> LYFQGAMALEEIKNGTDISTLDIRKFNLNINNVSVLSKSQSVDQFHLSNPHYEYLSGGAYPGEMENFTLKVDKSKKQDQVFENPLSLKFTNIGTVNGKQVDAYLNFNKVTLHYLNTAQAESEMNSAQKSTVEFFSISELWESNAFEIGNVPYVDANHDYIMNKAFWIDADVTAEIRYADGTETDLKLVMKPTDIDAIDANNLKETFYVKNYQNDVNLRLMNNANVLVQEEASDRTSWIATQITGGSYNENNVSGLALRSNSNSMNFGYSSTETCSAVFGLYIEKIDPRPVLEVDPAEIPAKDGQDVTYKATFKVPVPGKDILAAPSSIEMVQKFDERLDYKELKVESGGVTLQEGRDYTIEKTGQTVTVKMTPEYLKGNSSSDIIITYKTATNKKVEEKGSEKIDNTVTLHVDNLSAPSNQVSTALLYEK;> PTTENLYFQGAMALEEIKNGTDISTLDIRKFNLNINNVSVLSKSQSVDQFHLSNPHYEYLSGGAYPGEMENFTLKVDKSKKQDQVFENPLSLKFTNIGTVNGKQVDAYLNFNKVTLHYLNTAQAESEMNSAQKSTVEFFSISELWESNAFEIGNVPYVDANHDYIMNKAFWIDADVTAEIRYADGTETDLKLVMKPTDIDAIDANNLKETFYVKNYQNDVNLRLMNNANVLVQEEASDRTSWIATQITGGSYNENNVSGLALRSNSNSMNFGYSSTETCSAVFGLYIEKIDPRPVLEVDPAEIPAKDGQDVTYKATFKVPVPGKDILAAPSSIEMVQKFDERLDYKELKVESGGVTLQEGRDYTIEKTGQTVTVKMTPEYLKGNSSSDIIITYKTATNKKVEEKGSEKIDNTVTLHVDNLSAPSNQVSTALLYEK;> IPTTENLYFQGAMALEEIKNGTDISTLDIRKFNLNINNVSVLSKSQSVDQFHLSNPHYEYLSGGAYPGEMENFTLKVDKSKKQDQVFENPLSLKFTNIGTVNGKQVDAYLNFNKVTLHYLNTAQAESEMNSAQKSTVEFFSISELWESNAFEIGNVPYVDANHDYIMNKAFWIDADVTAEIRYADGTETDLKLVMKPTDIDAIDANNLKETFYVKNYQNDVNLRLMNNANVLVQEEASDRTSWIATQITGGSYNENNVSGLALRSNSNSMNFGYSSTETCSAVFGLY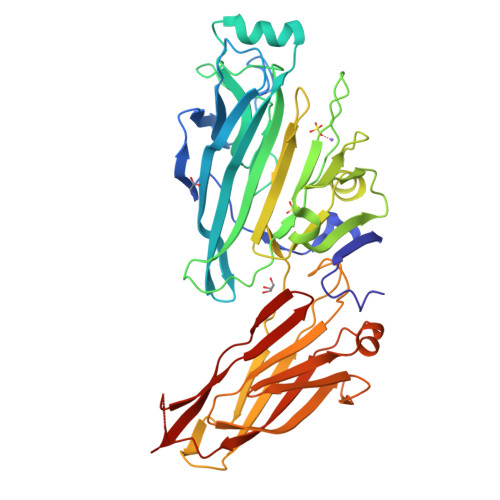IEKIDPRPVLEVDPAEIPAKDGQDVTYKATFKVPVPGKDILAAPSSIEMVQKFDERLDYKELKVESGGVTLQEGRDYTIEKTGQTVTVKMTPEYLKGNSSSDIIITYKTATNKKVEEKGSEKIDNTVTLHVDNLSAPSNQVSTALLYEK;> ALEEIKNGTDISTLDIRKFNLNINNVSVLSKSQSVDQFHLSNPHYEYLSGGAYPGEMENFTLKVDKSKKQDQVFENPLSLKFTNIGTVNGKQVDAYLNFNKVTLHYLNTAQAESEMNSAQKSTVEFFSISELWESNAFEIGNVPYVDANHDYIMNKAFWIDADVTAEIRYADGTETDLKLVMKPTDIDAIDANNLKETFYVKNYQNDVNLRLMNNANVLVQEEASDRTSWIATQITGGSYNENNVSGLALRSNSNSMNFGYSSTETCSAVFGLYIEKIDPRPVLEVDPAEIPAKDGQDVTYKATFKVPVPGKDILAAPSSIEMVQKFDERLDYKELKVESGGVTLQEGRDYTIEKTGQTVTVKMTPEYLKGNSSSDIIITYKTATNKKVEEKGSEKIDNTVTLHVDNLSAPSNQVSTALLYEK>[2x]AEAAKPATAADSKAAFKNDDQKSAYALGASLGRYMENS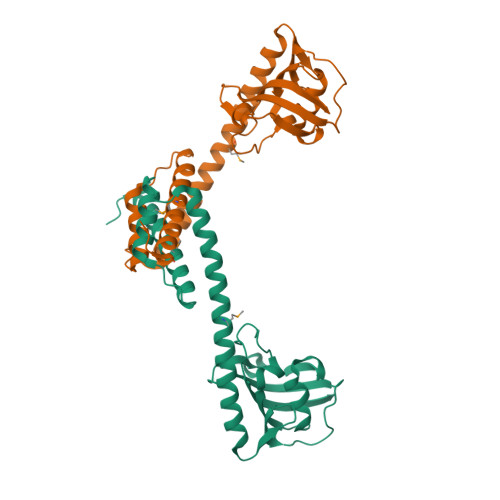LKEQEKLGIKLDKDQLIAGVQDAFADKSKLSDQEIEQTLQAFEARVKSSAQAKMEKDAADNEAKGKEYREKFAKEKGVKTSSTGLVYQVVEAGKGEAPKDSDTVVVNYKGTLIDGKEFDNSYTRGEPLSFRLDGVIPGWTEGLKNIKKGGKIKLVIPPELAYGKAGVPGIPPNSTLVFDVELLDVK advantame | C24 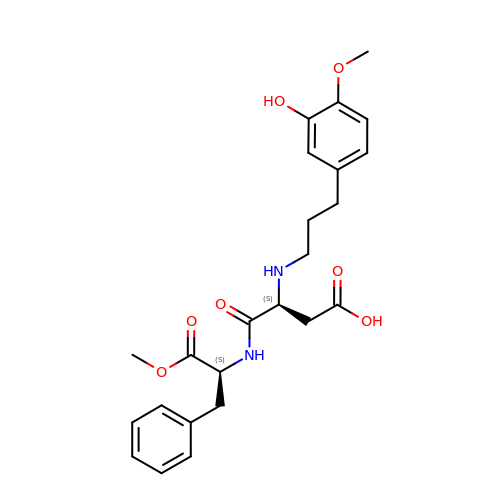H30 N2 O7 | YTKBWWKAVMSYHE-OALUTQOASA-N> SLMERLGGGGFSARIFVGLNVGDKPTYTIEDVVKDTIAIRKRQGILPDASFVAQRGVYTEQRSGQLVTENSVQIIIIDLEGLSKEDFTGKVQALGKELREDFKQESVIVEIQERGIVQDVYSITAEWYEEGPMRPLRVDLQPSLIS

Svi3-3 represents the first structure of a phage-encoded SAM degrading enzyme. Svi3-3 forms a trimer of ferredoxin-like fold alpha–beta sandwiches, where each subunit has two helices on the outside and a five-stranded anti-parallel beta sheet at the center. The subunits pack in a triangular manner, forming continuous beta sheets with their neighbors and are each in a ‘velcro-like’ topology where residues 2–6 at the N terminus of one subunit form beta-sheet interactions with residues 120–124 in β8 of another subunit. Prompted by DFT calculations producing high energy barriers for a hydrolysis reaction within the active site of Svi3-3, the TLC assays and NMR show unambiguously that Svi3-3 is a SAM lyase forming homoserine lactone and MTA.

Crystallization in the absence of ligands led to a lower-resolution apo structure. The structure of Svi3-3 in apo state is overall very similar to the complex structures (RMSD of 0.84 Å over 124 Cα atoms), but there is a shift of the N terminus, a conformational change of residues 7–9 to form a more extensive interaction with β9 and the preceding loop of the neighboring subunit, leading to a slight loosening of the trimer. In addition, residues 64 and 65 in the β5–β6 hairpin are disordered. Small angle X-ray scattering (SAXS) data confirmed that Svi3-3 has a similar trimeric structure in apo state as in the presence of SAM, indicating that product release and substrate binding do not require trimer dissociation. Svi3-3 forms a trimer in solution both in the absence and in the presence of substrate. Comparisons of the apo and ligand-bound structures as well as MD simulations indicate that stabilization is caused by tightening of the trimer around the ligand. Comparison of the average root mean square fluctuation (RMSF) of the protein backbone shows that Svi3-3 is more flexible throughout the 100 ns MD simulation in apo state (RMSF for trimer 0.91 Å2) than with SAM in the active site (RMSF for trimer 0.86 Å2). Interestingly, the residues surrounding the active site cavity, and in particular the methionine-stabilizing residues 104–106, become significantly more flexible in the apo simulations. Thus, 100 ns of MD simulation demonstrated that apo Svi3-3 shows the highest flexibility in the regions surrounding the active site, and that these regions become significantly more rigid upon substrate binding.AP sites are then processed by apurinic/apyrimidinic endonuclease 1 (APE1), which cleaves the phosphodiester DNA backbone at the 5′ end of the AP site using its endonuclease activity. Upon binding an AP site, APE1 flips the AP site out of the DNA double helix and into an extrahelical position within the compact APE1 active site. In the human APE1 substrate complex, N174 is within hydrogen bonding distance of N212 and the AP site bridging oxygen (O5) and deoxyribose sugar oxygen (O4). To assess the role of N174 during APE1 catalysis, we rationally designed four mutations of N174: N174A, N174D, N174Q, and N174K.

We next crystallized APE1N174A with the same AP DNA in the presence of MnCl2, promoting APE1 cleavage of the AP site. From these crystals, we obtained a 1.97 Å structure of the APE1N174A mutant product complex in the P1 space group. Within the active site of the APE1N174A product complex, there is clear density for the cleaved DNA backbone and bound Mn2+. We overlayed the APE1N174A mutant product complex with the APE1WT product complex and observed similar active site conformations (RMSD = 0.208 of 2449 atoms). An exception was active site residue N212, which was positioned differently in the APE1N174A mutant compared to APE1WT. In the APE1N174A mutant, N212 fails to make this rotameric shift and remains in the same position as in the substrate structure. Hydrogen bonding is absent in the APE1N174A mutant, resulting in a 1.6 Å shift of the 5′ phosphate terminus away from residue N174A compared to WT. In the APE1N174A mutant, residue 174 cannot act as a steric barrier due to its reduced side chain length, resulting in a shift of over 2 Å away from the active site metal ion. In APE1WT, the 3′ hydroxyl is 2.1 Å from its metal cofactor, but this distance increases to 4.4 Å in the APE1N174A mutant. This finding indicates that in APE1WT, the side chain size of N174 acts as a steric barrier that, along with hydrogen bonding, properly positions the AP site within the APE1 active site for cleavage.

>[2x]ALYEDPPDQKTSPSGKPATLKICSWNVDGLRAWIKKKGLDWVKEEAPDILCLQETKCSENKLPAELQELPGLSHQYWSAPSDKEGYSGVGLLSRQAPLKVSYGIGDEEHDQEGRVIVAEFDSFVLVTAYVPAAGRGLVRLEYRQRWDEAFRKFLKGLASRKPLVLCGDLNVAHEEIDLRNPKGNKKNAGFTPQERQGFGELLQAVPLADSFRHLYPNTPYAYTFWTYMMNARSKNVGWRLDYFLLSHSLLPALCDSKIRSKALGSDHCPITLYLAL>MTLFPVLNNTPVGKQVDSIYESRLDQFLSEGQYRDFNLPSVYDHARIDNPSGDVNNDLSKGFVDLKVYRVPDLSRPSFNEVVGHKKFDETASKGDTFGPSWATFWFEVHIRLPKSWAKYEQVIFQWNCDNEGLVYSQDGVPLQAFSGSERTDFILPDSWKTTE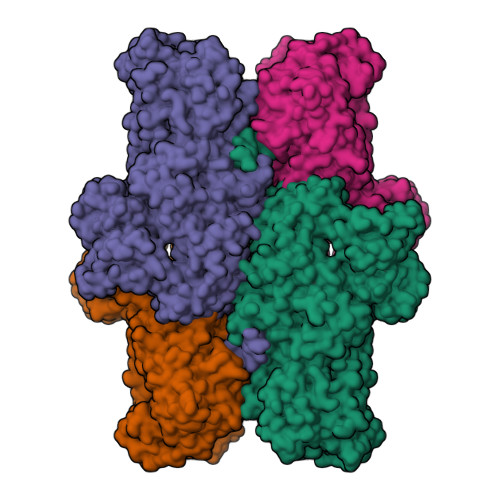DTFYIEMACNGMFGTGAGSQIAPPDPNRYFTLTKADLVAPNLPAMALAYDFLLMQQCVKQLPSNCWQKYKARQICNDIMNTFHPNDLSTINECRNLAKAFLGNDIDSEAVFEKNNDKANVFAIGHCHIDTAWLWPFAETRRKIVRSWATQMNIMDRYPEYQFVCSQALQYLWLKEDHPDVFEKLKEYVNQNKFIPIGGSWVEHDTNIPNGESLIRQFLLGQHFFEKEFGVRCRTFWLPDTFGYSSQIPQICRLCGMDRFLTQKLSWNNINSFPTSTFNWVALDGSQVICHMPPANTYTADTNVNDVLHSIDQHKNLVNDQAGLLVFGIGDGGGGPTPEMLEKLRRCKGIANTVGYLPNVKLGNTVDEFFDGILKRTNAGQTLPSWNGELYFEFHRGTYTTQAELKKLMRKVEIALHDAEYVSTLASIFSKDYSYPKESLQDLWRDTLLCQFHDVLPGSCIEMVYKDAIPIMSKVLKNTEALLWQAIEQLGFKKASSSDNKEQLCLLNTLPWNVRGVITETEENKLVYFESCDGKGILTAAHTSLKHPAAAYQKDDNFILVNDHLRVTIAPNGLILSLFDLHKEREILDLKSGKNHAGANQYVLFEDTPLSWQAWDTEVFSLEKYEVLDKGKVSIKESGPLRASVVVDIPISELSHMKATISLEGYNDCSEFTGVNFTCEVDWHESCKFLKVEFPVDIHSEFASYETQFGITKRPTHYNTSWDVAKFEVCHQKFADYSDFTYGVSVLNDCKYGFSTHGNLMRLSLLRSPKQPDAHADMGKHTIRYAVYPHSKPLDSSTVRAAHKFNSNFRLLTRASDTANLDIFDAFQLVGEPNVILSHIKMAEKGKSIILRVYESLGGKSRARLVIKSLTVASVTKCNGLEEDLEELCTLKSNDYYEVPIELRAFEIATFKVNLGSMSKGKVVDIMDYKDDDDKPMDYKDDDDKHHHHHHDELYKRSGAPLLNKRISYDL[4x]>[4x]MTKYTYPATLLCDFYKVSHKEQYPEGTELIYSTWTPRTSRVEDIDRVVAFGFQGFIKKYLIDYFNENFFKRPKQDVVNEYKRVIKHTLQVDDPDASHIESLHELGYLPIKIKAVKEGTFIPIKVPMLTIENTIPEFFWITNYLETLMSNEIWQPTTSATLAYEYRKILDEYAMETVGNKLAVDFQGHDFSMRGMSSLESTKLSGAGHLLSFTGTDTIPAILYHE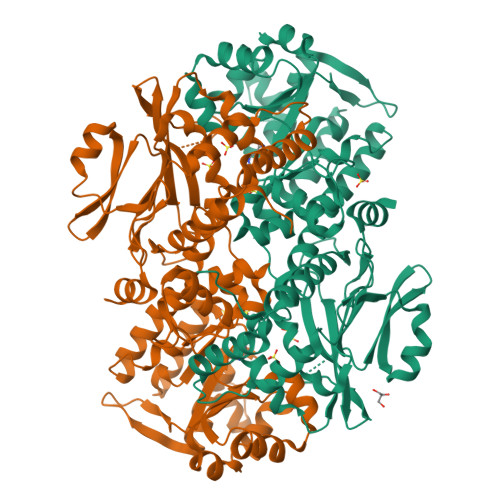EFYNANIENELVGSSIPATEHSVMCANGQDEYVVFKKLITETYPEGFVSIVSDTWDFWNVIDTVVRKLKGDILKRDGKVVIRPDSGDPVKIICGDPEAKDELVRKGLIEVLWDIFGGNVTDKGYKVLDPHIGAIYGDAITISRCKEICKKLAAKGFASVNVVFGIGSFTYQYNTRDTFGFAMKATYTVVNGEERQIFKNPKTDDGTKKSQKGLVAVVNNGNELSLVDELDRNAYKQLSNDDILEDVFINGQLLRNQTLSEIRELLLD>[4x]MASLTLNTVKQIFRAMADSPGFDRVLSKVEVLSAAPGKVVCEMKVEEQHTNRGGTLHGGMTATLVDMISTMAIMYSERGAPGVSVDMNITYMNAAKIGEDILITAQVLKQGRTLAFAT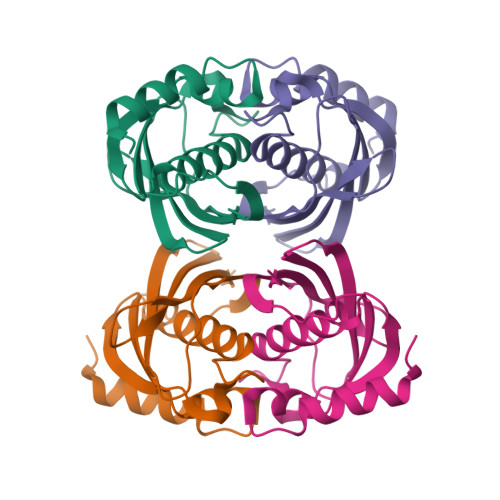VDLTNKANGKLIAQGRHTKHLGSLEHHHHHH> GPSFREQDIYLPIANVARIMKNAIPQTGKIAKDAK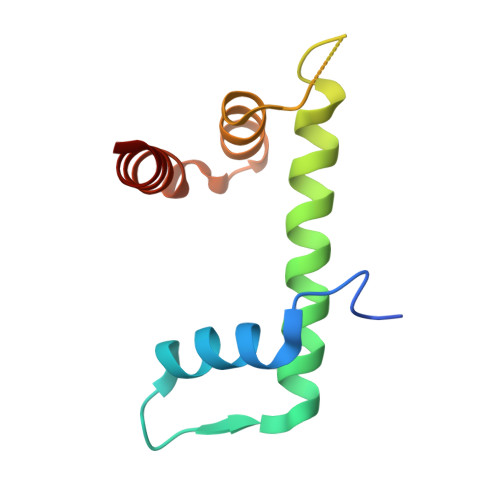ECVQECVSEFISFITSEASERCHQEKRKTINGEDILFAMSTLGFDSYVEPLKLYLQKFRE SK catalyzes the specific phosphorylation of the 3-hydroxyl group of shikimic acid, using ATP as a co-substrate. The shikimate pathway is comprised of seven enzymatic components that convert erythrose 4-phosphate and phosphoenolpyruvate into chorismate, for subsequent synthesis of aromatic compounds. SKs belong to a class of P-loop kinases that share a homologous α-β-α fold. Overall, these structures have a characteristic α-β-α fold that consists of the CORE domain (residues 1–31, 61–108, and 124–162), the SB domain (residues 32–60), and the LID region (residues 109–123) in the monomer.

The HpSK•S3P•ADP structure shows clear electron density for all residues. Within the binding pocket, there is a large piece of non-peptide density that can easily be modeled as the product S3P, and nearby density can be built as ADP. The LID region covers the binding pocket in which the guanidino group of R116 has direct contacts with S3P and the β-phosphate of ADP, forming strong hydrogen bonds. Based on these structures, it is likely that S3P is chelated by R57 and R132 via a hydrogen-bonding network in HpSK•shikimate•PO4 and HpSK•S3P•ADP. This would lead to a small movement in the peptide backbone, propagated through the α6 helix into the adjacent LID loop. A subsequent large conformational rearrangement of this loop would allow the side chain of R116 to bind to the phosphate group of S3P, as seen in HpSK•S3P•ADP, or possibly the γ-phosphate moiety of ATP. Superposition of HpSK• S3P•ADP and E114•162535 shows that only R57 and R132 stay at approximately the same position; M10 and R116 are situated at rather distinct positions to interact with S3P and NSC162535, respectively. Additionally, HpSK•S3P•ADP and E114•162535 have different contacting residues, (D33, V44, G79, P117, L118, and F9, R45, F48, V83, M84, L135, Y136, respectively). In the HpSK•S3P•ADP state, NSC162535 docked into a site where there were no direct contacts with the Nη1 and Nη2 atoms of R116.

> HHHHHHMQHLVLIGFMGSGKSSLAQELGLALKLEVLDTDMIISERVGLSVREIFEELGEDNFRMFEKNLIDELKTLKTPHVISTGGGIVMHENLKGLGTTFYLKMDFETLIKRLNQKEREKRPLLNNLTQAKELFEKRQALYEKNASFIIDARGGLNNSLKQVLQFIA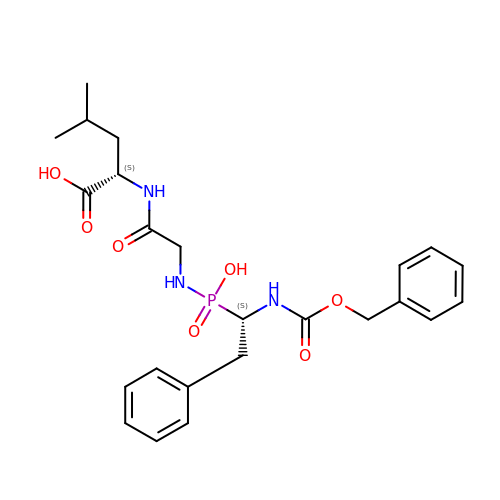(2~{S})-4-methyl-2-[2-[[oxidanyl-[(1~{S})-2-phenyl-1-(phenylmethoxycarbonylamino)ethyl]phosphoryl]amino]ethanoylamino]pentanoic acid | C24 H32 N3 O7 P | YJSHTZYDPJRJOL-UNMCSNQZSA-N> MNNNKAEADTSSSMADPETRPTYTTHHLAIPSGVTQDEFDELKQSVVEFH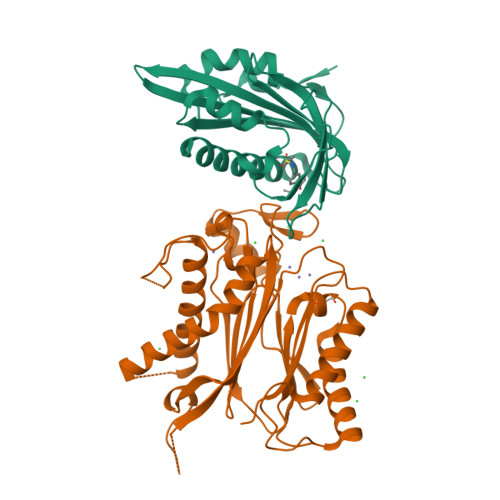TYQLSQNQCSSLLAQRIRAPNDVVWSIVRRFDQPQTYKHFIKSCSVSDNFTMAVGSTRDVNVISGLPAATSTERLDILDDDRQVTGFSIIGGEHRLRNYRSVTSVHGFNRDGAICTVVLESYVVDVPEGNTEEDTRLFADTVVKLNLQKLVSVAESQVI;> RSVYELDCIPLWGVVSIQGNRSEMEDAFAVSPHFLKLPIKMLMGDHAGMSPSLTHLTGHFFGVYDGHGGHKVADYCRDRLHFALAEEIERIKDELCKRNTGEGRQVQWDKVFTSCFLTVDGEIEGKIGRAVVGSSDKVLEAVASETVGSTAVVALVCSSHIVVSNCGDSRAVLFRGKEAMPLSVDHKPDREDEYARIENAGGKVIQWQGARVFGVLAMSRSIGDRYLKPYVIPEPEVTFMPRSREDECLILASDGLWDVMNNQEVCEIARRRILMWHKKNGAPPLAERGKGIDPACQAAADYLSMLALQKGSKDNISIIVIDLKAQRKFKTRT> NAHNF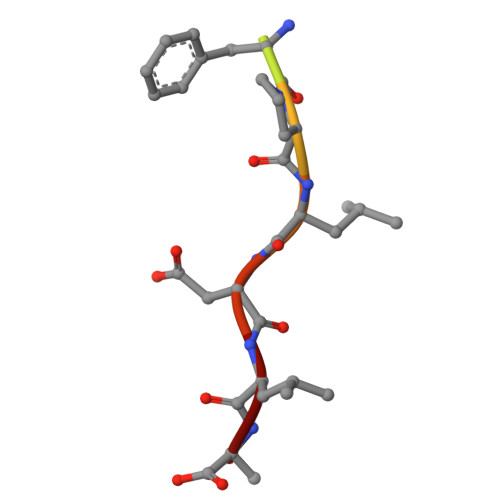PLDLA>[4x]GHMSRNLLAIVHPILRNLMEESGE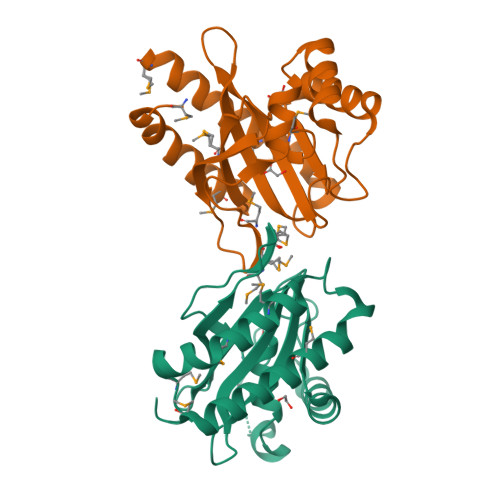TVNMAVLDQSDHEAIIIDQVQCTHLMRMSAPIGGKLPMHASGAGKAFLAQLSEEQVTKLLHRKGLHAYTHATLVSPVHLKEDLAQTRKRGYSFDDEEHALGLRCLAACIFDEHREPFAAISISGPISRITDDRVTEFGAMVIKAAKEVTLAYGGMRGS> MKLDIKKTFSNRSDRVKGIDFHPTEPWVLT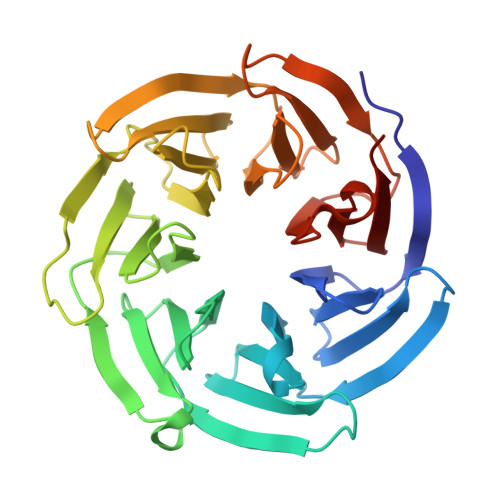TLYSGRVELWNYETQVEVRSIQVTETPVRAGKFIARKNWIIVGSDDFRIRVFNYNTGEKVVDFEAHPDYIRSIAVHPTKPYVLSGSDDLTVKLWNWENNWALEQTFEGHEHFVMCVAFNPKDPSTFASGCLDRTVKVWSLGQSTPNFTLTTGQERGVNYVDYYPLPDKPYMITASDDLTIKIWDYQTKSCVATLEGHMSNVSFAVFHPTLPIIISGSEDGTLKIWNSSTYKVEKTLNVGLERSWCIATHPTGRKNYIASGFDNGFTVLSLGNDE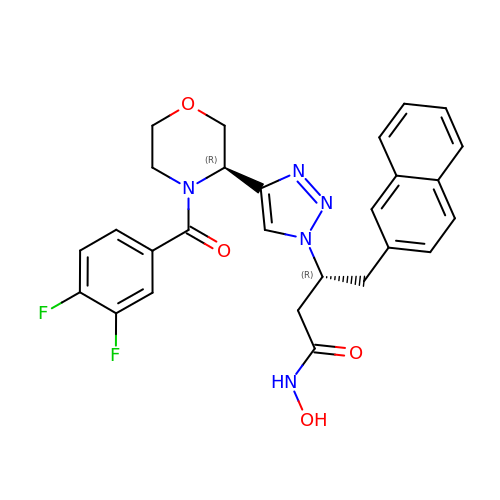(3R)-3-{4-[(3R)-4-(3,4-difluorobenzene-1-carbonyl)morpholin-3-yl]-1H-1,2,3-triazol-1-yl}-N-hydroxy-4-(naphthalen-2-yl)butanamide | C27 H25 F2 N5 O4 | DDQJIEMCJUWZNL-BWKNWUBXSA-N> MGKRVLIVDDAAFMRMMLKDIITKAGYEVAGEATNGREAVEK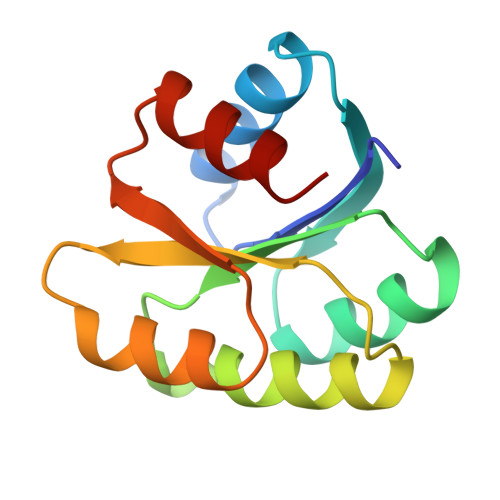YKELKPDIVTMDITMPEMNGIDAIKEIMKIDPNAKIIVCSAMGQQAMVIEAIKAGAKDFIVKPFQPSRVVEALNKVSK>[4x]MRTIHANSSAVREDHRALDVATELAKTFRVTVRERERAGGTPKAERDAIRRSGLLTLLISKERGGLGESWPTVYEAIAEIASADASLGHLFGYHFSNFAYVDLFASPEQKARWYPQAVRERWFLGNASSENNAHVLDWRVTATPLPDGSYEINGTKAFCSGSADA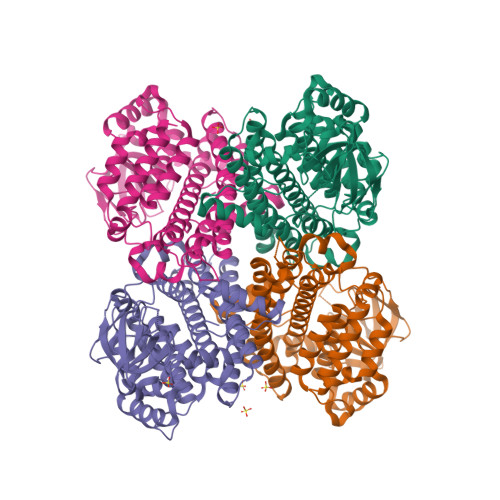DRLLVFAVTSRDPNGDGRIVAALIPSDRAGVQVNGDWDSLGMRQTDSGSVTFSGVVVYPDELLGTPGQVTDAFASGSKPSLWTPITQLIFTHLYLGIARGALEEAAHYSRSHSRPFTLAGVEKATEDPYVLAIYGEFAAQLQVAEAGAREVALRVQELWERNHVTPEQRGQLMVQVASAKIVATRLVIELTSRLYEAMGARAAASRQFGFDRFWRDARTHTLHDPVAYKIREVGNWFLNHRFPTPSFYS(2R,3R,3aS,5R,7aR,9R,10R,10aS,12R,14aR)-2,9-bis(6-amino-9H-purin-9-yl)octahydro-2H,7H-difuro[3,2-d:3',2'-j][1,3,7,9,2,8]tetraoxadiphosphacyclododecine-3,5,10,12-tetrol 5,12-dioxide | C20 H24 N10 O12 P2 | 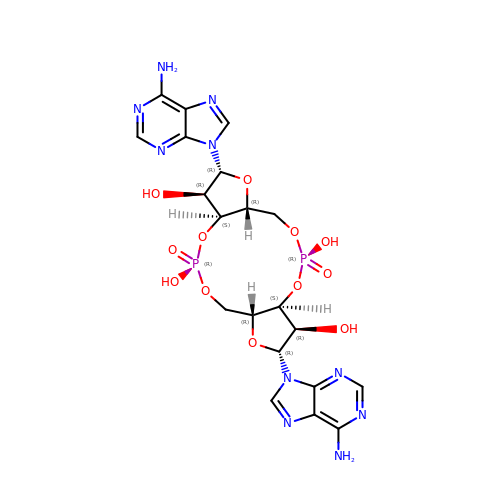PDXMFTWFFKBFIN-XPWFQUROSA-N> AYFAGMRPLHPIDFIFLSLEKRQQPMHVGGLFLFQIPDNAPDTFIQDLVNDIRISKSIPVPPFNNKLNGLFWDEDEEFDLDHHFRHIALPHPGRIRELLIYISQEHSTLLDRAKPLWTCNIIEGIEGNRFAMYFKIHHAMVDGVAGMRLIEKSLSHDVTEKSIVPPWCVEGKRAKRLREPKTGKIKKIMSGIKSQLQATPTVIQELSQTVFKDIGRNPDHVSSFQAPCSILNQRVSSSRRFAAQSFDLDRFRNIAKSLNVTINDVVLAVCSGALRAYLMSHNSLPSKPLIAMVPASIRNDDSDVSNRITMILANLATHK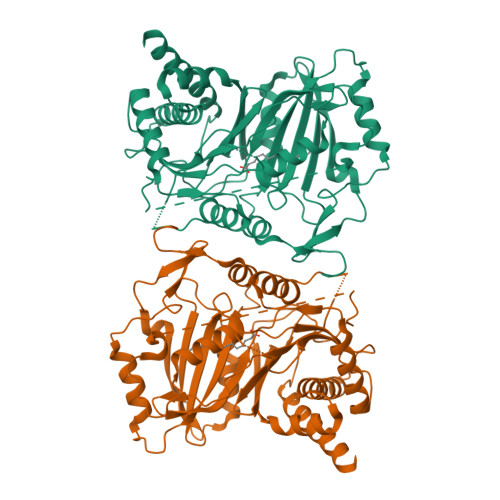DDPLQRLEIIRRSVQNSKQRFKRMTSDQILNYSAVVYGPAGLNIISGMMPKRQAFNLVISNVPGPREPLYWNGAKLDALYPASIVLDGQALNITMTSYLDKLEVGLIACRNALPRMQNLLTHLEEEIQLFEGVIAKQEDIKTAN>SNAAKDVKFGADARALMLQGVDLLADAVAVTMGPKGRTVIIEQSWGSPKVTKDGVTVAKSIDLKDKYKNIGAKLVQDVANNTNEEAGDGTTTATVLARSIAKEGFEKISKGANPVEIRRGVMLAVDAVIAELKKQSKPVTTPEEIAQVATISANGDKEIGNIISDAMKKVGRKGVITVKDGKTLNDELEIIEGMKFDRGYISPYFINTSKGQKCEFQDAYVLLSEKKISSIQSIVPALEIANAHRKPLVIIAEDVDGEALSTLVLNRLKVGLQVVAVKAPGFGDNRKNQLKDMAIATGGAVFGEEGLTLNLEDVQPHDLGKVGEVIVTKDDAMLLKGKGDKAQIEKRIQEIIEQLDVTTSEYEKEKLNERLAKLSDGVAVLKVGGTSDVEVNEKKDRVTDALNATRAAVEEGIVLGGGCALLRCIPALDSLTPANEDQKIGIEIIKRTLKIPAMTIAKNAGVEGSLIVEKIMQSSSEVGYDAMAGDFVNMVE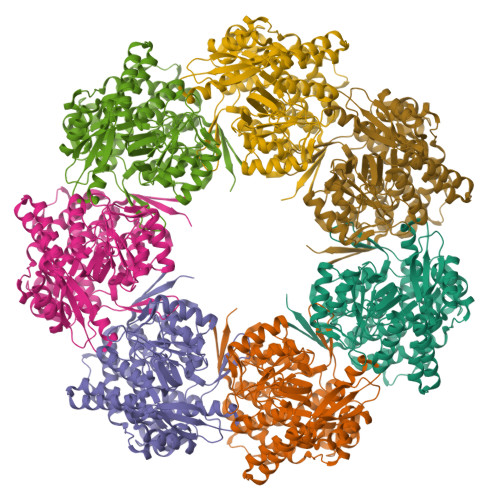KGIIDPTKVVRTALLDAAGVASLLTTAEVVVTEIPKEEKDPGMGAMGGMGGGMGGGMF[7x]>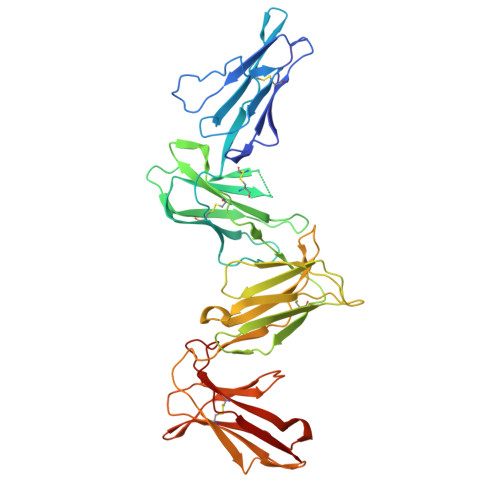 GIQPKPTLWAEPDSVITQGSPVTLSCQGSLEAQEYRLYREKKSASWITRIRPELVKNGQFHIPSITWEHTGRYGCQYYSRARWSELSDPLVLVMTGAYPKPTLSAQPSPVVTSGGRVTLQCESQVAFGGFILCKEGEEEHPQCLNSQPHARGSSRAIFSVGPVSPNRRWSHRCYGYDLNSPYVWSSPSDLLELLVPGVSKKPSLSVQPGPVMAPGESLTLQCVSDVGYDRFVLYKEGERDLRQLPGRQPQAGLSQANFTLGPVSRSYGGQYRCYGAHNLSSECSAPSDPLDILITGQIRGTPFISVQPGPTVASGENVTLLCQSWRQFHTFLLTKAGAADAPLRLRSIHEYPKYQAEFPMSPVTSAHAGTYRCYGSLNSDPYLLSHPSEPLELVVS> MSSTVISRKRRNSTVTEPDSSGETRKQKKSRSDEKSSSSKDGDPQLEFKVLQGYRDLESEMHKGRAQVTRTGDIGVAMDNLNAVDSLFNKVIGIKNNGLFAHDARAMVSISELAQISVRNLKFDDSRSMVNLENIVNSLKRYMLKEHFKLNNIAENRNDLTLAADEQSAADQQEESDGDIDRTPDDNHTDKATSSFKATSMRHSYLQQFSHYNEFSQFNWFRIGALYNTISKNAPITDHLMGPLSIEKK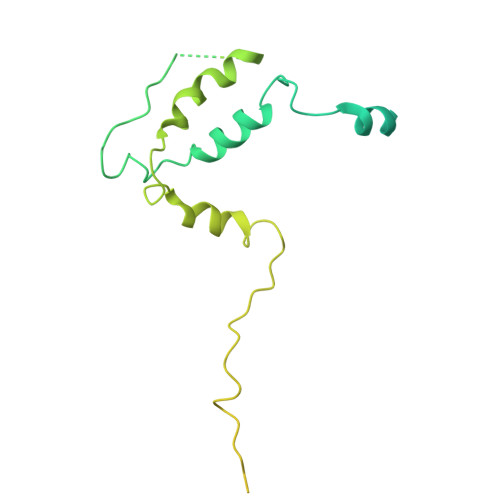PRVLTQRRRNNDQVGEKITAEKITQHSLNSTQQETTPEQVKKCFKKLSKKLGPEGSINLFKFIIDPNSFSRSIENLFYTSFLIKEGKLLMEHDEEGLPTIKIKQSISHTDSRSKEIERQRRRAAHQNHIIFQMDMPTWRKLIKKYNITSPFLD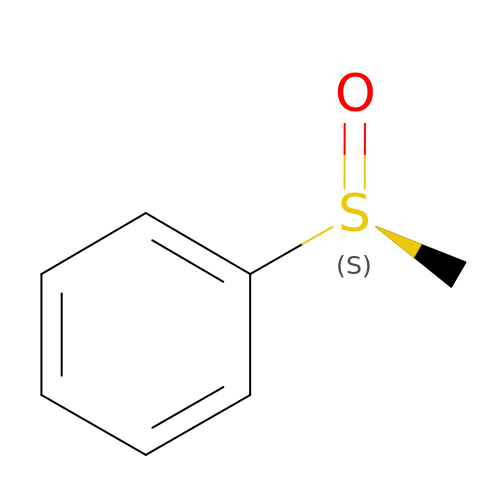[(S)-methylsulfinyl]benzene | C7 H8 O S | JXTGICXCHWMCPM-VIFPVBQESA-N>[6x]MNKFKVNISGMTCTGCEKHVESALEKIGAKNIESSYRRGEAVFELPDDIEVESAIKAIDEANYQAGEIEEVSSLENVALINEDNYDLLIIGSGAAAFSSAIKAIEYGAKVGMIERGTVGGTCVNIGCVPSKTLLRAGEIIHLSKDNPFIGLQTSAGEVDLASLITQKDKLVSELRNQKYMDLIDEYNFDLIKGEAKFVDASTVEVNGAKLSAKRFLIATGASPSLPQISGLEKMDYLTSTTLLELKKIPKRLTVIGSGYIGMELGQLFHHLGSEITLMQRSERLLKEYDPEISESVEKALIEQGINLVKGATFERVEQSGEIKRVYVTVNGSREVIESD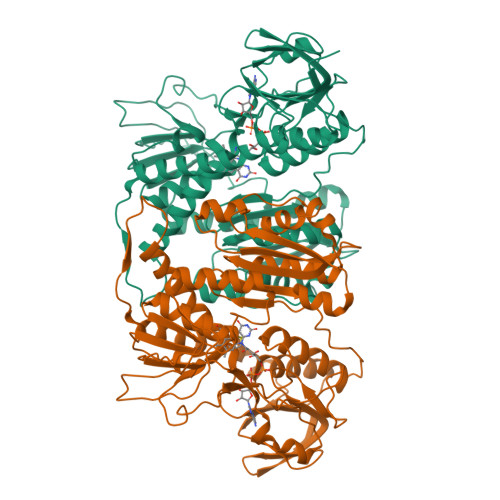QLLVATGRKPNTDSLNLSAAGVETGKNNEILINDFGQTSNEKIYAAGDVTLGPQFVYVAAYEGGIITDNAIGGLNKKIDLSVVPAVTFTNPTVATVGLTEEQAKEKGYDVKTSVLPLDAVPRAIVNRETTGVFKLVADAETLKVLGVHIVSENAGDVIYAASLAVKFGLTVEDLTETLAPYLTMAEGLKLAALTFDKDIWKLSCCAGLEHHHHHH[[(3R,4R,5S,6R)-3-acetamido-4,5-bis(oxidanyl)-6-(sulfooxymethyl)oxan-2-ylidene]amino] 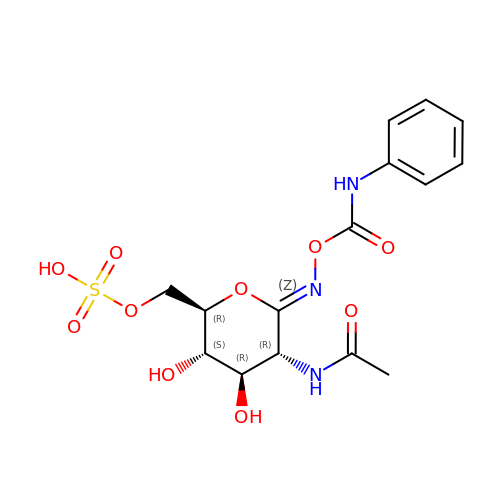N-phenylcarbamate | C15 H19 N3 O10 S | CQRQAZDSYYFJGD-FDYHWXHSSA-N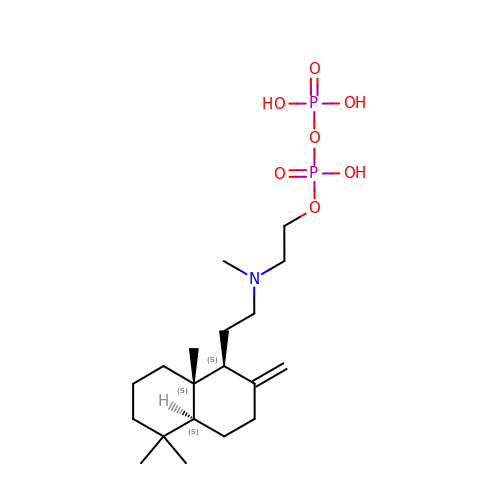2-(methyl{2-[(1S,4aS,8aS)-5,5,8a-trimethyl-2-methylidenedecahydronaphthalen-1-yl]ethyl}amino)ethyl trihydrogen diphosphate | C19 H37 N O7 P2 | ZYKKZQANNLZNRN-JENIJYKNSA-N>[2x]HHHHHHFNLPPGNYKKPVLLYCSNGGHFLRIDPAGTVDGTRDRSDQHIQLQLSAESVGEVYIKSTETGQYLAMDTDGLLYGSQTPNEE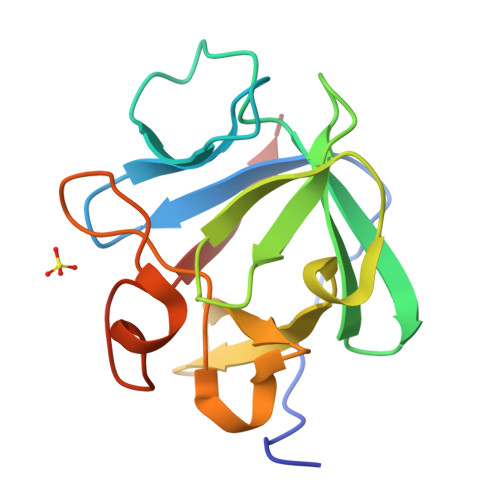CLFLERLEENHYNTYISKKHAEKNWFVGLKKNGSCKRGPRTHYGQKAILFLPLPVSSD2-[(carboxymethyl)amino]benzoic 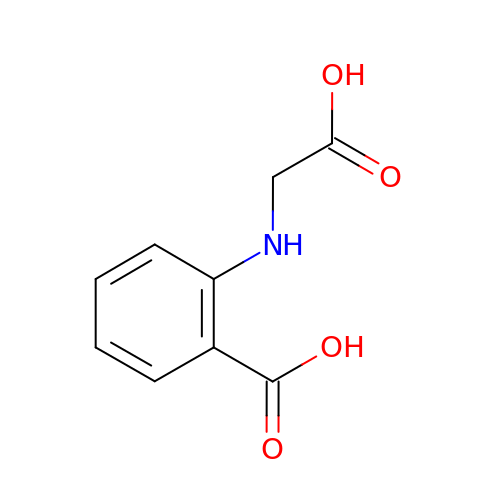acid | C9 H9 N O4 | PJUXPMVQAZLJEX-UHFFFAOYSA-N> GPVEDAVTAAIGRVADTVGTGPTNSEAIPALTAAETGHT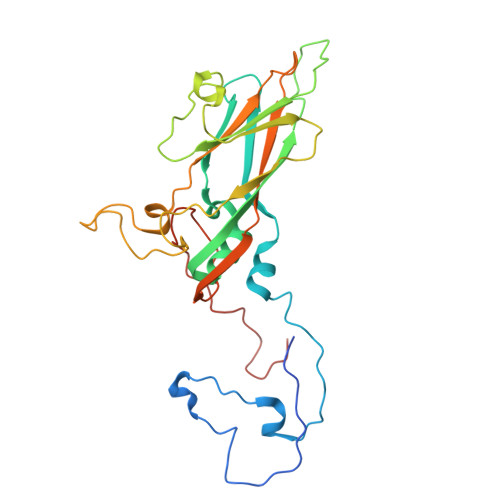SQVVPGDTMQTRHVKNYHSRSESTVENFLCRSACVYFTEYKNSGSKRYAEWVVTTRQAAQLRRKLEFFTYIRFDLELTFVITSTQQPSTTQNQDAQILTHQIMYVPPGGPVPDKVDSYVWQTSTNPSVFWTEGNAPPRMSIPFLSIGNAYSNFYDGWSDFSRDGVYGINTLNSMGTLYARHVNTGGTGPIKSTIRIYFKPKHVKAWIPRPPRLCQYEKAKNVNFQPSGVTTTRQSITAMTNTGAF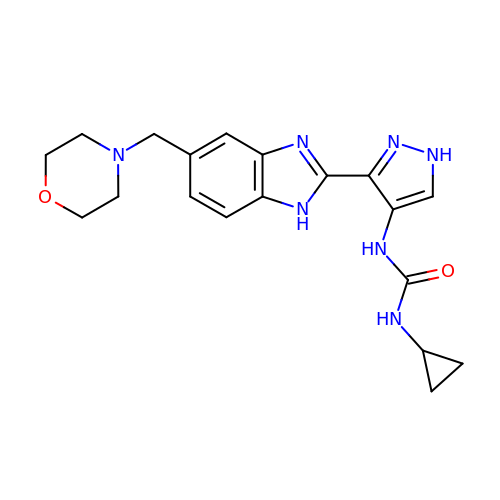1-cyclopropyl-3-{3-[5-(morpholin-4-ylmethyl)-1H-benzimidazol-2-yl]-1H-pyrazol-4-yl}urea | C19 H23 N7 O2 | LOLPPWBBNUVNQZ-UHFFFAOYSA-N> GSLVLYGAPYAAAVEVLEETLRETGARYALLIDRKGFVLAHKEALWAPKPPPLDTLATLVASNAAATQALAKLLGEARFQEEVHQGERMGLYVDEAGEHALLVLVFDETAP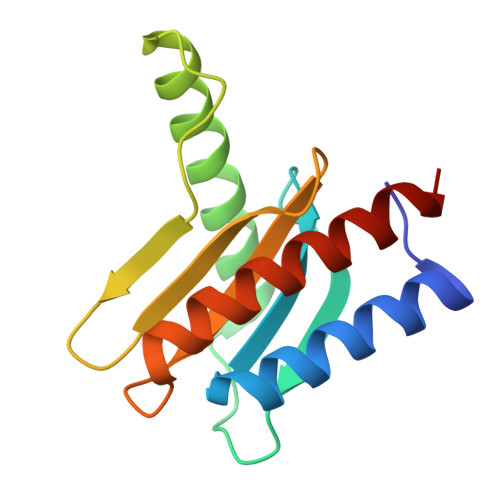LGKVKLHGKAAAAALAAIAEEALAN5-thio-alpha-D-mannopyranosylamine | 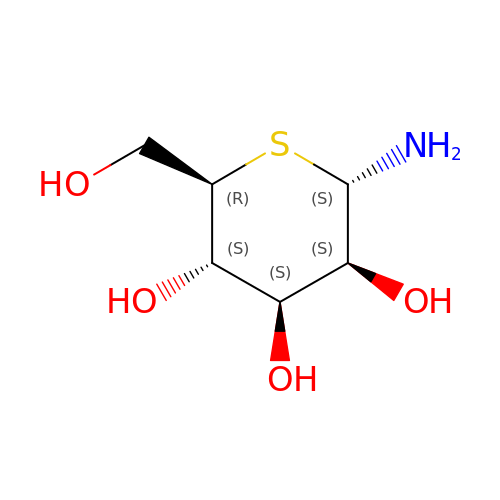C6 H13 N O4 S | FGVRMLQUWLZGLJ-PQMKYFCFSA-N>[4x]MKKNHHHHHHLVPRGSKLA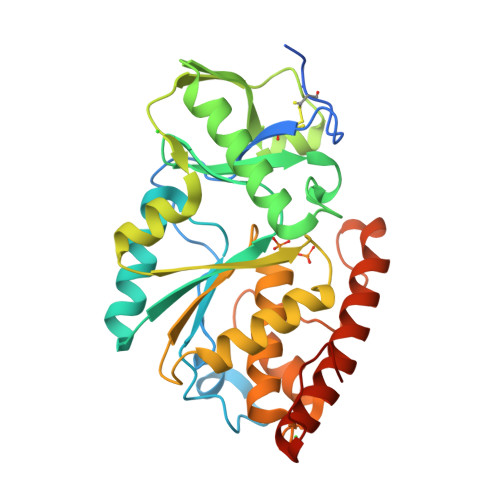SSIVCDSTIENPCIVQDSKTQFSPVIRYREVASIADVYGGNITGINKFHLSGSEQPSEKGWEAIAESISRKMGAETKKVIVLDLRQESHGYLNGRAITLVSAYNWINLGKSNSQSTLDQENWLAGLRSRKIVNGVLTVPQYVAKQYSQGKSMVVSTVKNEEYYVYKKGFDYYRIFISDHRAPLDSEVDALVALIKNNPEDTWYHVHCRGGKGRTTTVFAMFDMLKNADKVSFEEIIARQASIPPFYNLMVTNREIPELTPYYEQRLQFLIHFYEFARQSLMGYSGTWSEWKKLNI>GSPNYDKWEMERTDITMKHKLGGGQYGEVYEGVWKKYSLTVAVKTLKEDTMEVEEFLKEAAVMKEIKHPNLVQLLGVCTRE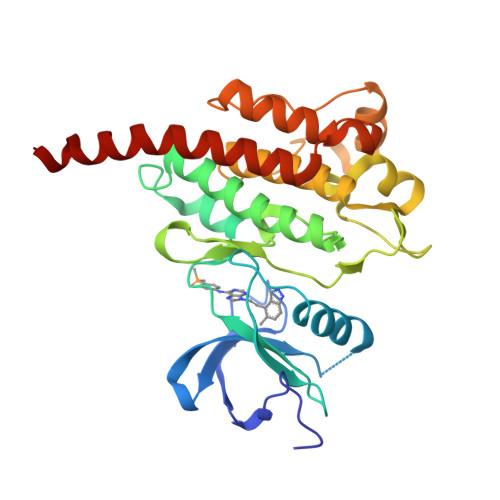PPFYIITEFMTYGNLLDYLRECNRQEVSAVVLLYMATQISSAMEYLEKKNFIHRDLAARNCLVGENHLVKVADFGLSRLMTGDTYTAHAGAKFPIKWTAPESLAYNKFSIKSDVWAFGVLLWEIATYGMSPYPGIDLSQVYELLEKDYRMERPEGCPEKVYELMRACWQWNPSDRPSFAEIHQAFETMFQESSISDEVEKELGKRGT[2x]RNA interference by type III CRISPR systems results in the synthesis of cyclic oligoadenylate (cOA) second messengers, which are known to bind and regulate various CARF domain–containing nuclease receptors. The CARF domain–containing Csa3 family of transcriptional factors associated with the DNA-targeting type I CRISPR systems regulate expression of various CRISPR and DNA repair genes in many prokaryotes. An atomic structure of the apo form of a Csa3a homolog from S. solfataricus (Csa3Sso) has been previously reported to harbor an N-terminal CARF and a C-terminal MarR-like winged helix-turn-helix (wHTH) domain. Here, we identify cA4 as the cognate ligand of Csa3Sso and show that Csa3Sso lacks ring nuclease activity in vitro.

To better understand the structural basis for Csa3Sso ligand specificity, we determined a 2.05-Å X-ray crystal structure of His6-Csa3Sso bound to cA4. Like the apo Csa3Sso structure, the Csa3Sso dimer is domain swapped with respect to an N-terminal CARF and the C-terminal wHTH DNA-binding domains of the two protomers A and B. Overall, these data evidence monodisperse dimers of Csa3Sso in solution that persist in the presence and absence of cA4. Consistent with in-solution dimers observed for Csa3Sso, the asymmetric unit for the Csa3Sso•cA4 complex structure consisted of a dimer of Csa3Sso bound to one molecule of cA4.Figure 3 cA4-bound Csa3Ssois a dimer in solution. Comparison of all the cA4-bound structures of CARF domain proteins revealed that cA4 in the Csa3Sso–cA4 complex structure exists in a unique elongated conformation. In this conformation, P1a and P1b (called distal phosphoryl groups) in the cA4 ring are stretched outward (with a P-to-P distance of 11.8 Å), which brings P2a and P2b (called proximal phosphoryl groups) to a shorter P-to-P distance of 4.4 Å. The hallmark of all the adenine-binding pockets in Csa3Sso are π-stacking interactions of Phe14A&B and Phe10A&B with the nonplanar (A1a and A1b) and planar (A2a and A2b) adenine rings, respectively. The inward-facing phosphoryl group in the middle of the elongated cA4 (P2b) was found to hydrogen bond with highly conserved Arg98A&B (cA4 binding motif 2) and Glu122A (β5–α5 loop) residues in Csa3Sso. Of interest, the cA4 phosphoryl interacting surface of the Csa3Sso pocket is largely positively charged except for the conserved Glu122 residue that hydrogen bonds with cA4 central phosphoryl (P2b) oxygen via its side-chain carboxyl in the protomer A. Such interactions of Glu122 side chains could create an electrostatic repulsion with central phosphoryls (P2a and P2b) likely constraining them close to each other in the elongated cA4 conformation. Also, the active site interactions of Arg98 and Glu122 with the target cA4 phosphoryl (P2b) results in an O’-P’-O” angle of 94° presenting with a stereochemistry inconducive for nucleophilic attack by the 2′ ribosyl hydroxyl.

>MHHHHHHHGAAMKSYFVTMGFNETFLLRLLNETSAQKEDSLVIVVPSPIVSGTRAAIESLRAQISRLNYPPPRIYEIEITDFNLALSKILDIILTLPEPIISDLTMGMRMINTLILLGIIVSRKRFTVYVRDEGGGSRVISFNDNTIRALMRDYSREEMKLLNVLYETKGTGITELAKMLDKSEKTLINKIAELKKFGILTQKGKDRKVELNELGLNVIKLNKSVIESSKSSEELVKENKGKEVNIPY[2x]>[2x]MYRTAASRARALKGVLTRSLRPARYASSSAVAETSSSTPAYLSWLSGGSRAALTSLDMPLQGVSLPPPLADKVEPSKLQITTLPNGLKIASETTPNPAASIGLYVDCGSIYEAPYFHGATHLLERMAFKSTLNRTHFRLVREIEAIGGNTSASASREQMSYTIDALKTYVPEMVEVLIDSVRNPAFLDWEVNEELRKMKVEIAELAKNPMGFLLEAIHSAGYSGPLASPLYAPESALDRLNGELLEEFMTENFTAARMVLAASGVEHEELLKVAEPLTSDLPNVPPQLAPKSQYVGGDFRQHTGGEATHFAVAFEVPGWNNEKEAVTATVLQMLMGGGGSFSAGGPGKGMHSWLYRRVLNEYQEVQSCTAFTSIFNDTGLFGIYGCSSPQFAAKAIELAAKELKDVAGGKVNQAHLDRAKAATKSAVLMNLESRMIAAEDIGRQILTYGERKPVDQFLKSVDQLTLKDIADFTSKVISKPLTMGSFGDVLAVPSYDTISSKFR;>[2x]MAMKNLLSLARRSQRRLFLTQATRSSSSFSAIDSVPASASPTALSPPPPHLMPYDHAAEIIKNKIKKLENPDKRFLKYASPHPILASHNHILSAPETRVTTLPNGLRVATESNLSAKTATVGVWIDAGSRFESDETNGTAHFLEHMIFKGTDRRTVRALEEEIEDIGGHLNAYTSREQTTYYAKVLDSNVNQALDVLADILQNSKFEEQRINRERDVILREMQEVEGQTDEVVLDHLHATAFQYTPLGRTILGPAQNVKSITREDLQNYIKTHYTASRMVIAAAGAVKHEEVVEQVKKLFTKLSSDPTTTSQLVANEPASFTGSEVRMIDDDLPLAQFAVAFEGASWTDPDSVALMVMQTMLGSWNKNVGGGKHVGSDLTQRVAINEIAESIMAFNTNYKDTGLFGVYAVAKADCLDDLSYAIMYEVTKLAYRVSDADVTRARNQLKSSLLLHMDGTSPIAEDIGRQLLTYGRRIPTAELFARIDAVDASTVKRVANKYIYDKDIAISAIGPIQDLPDYNKFRRRTYWNRY;>[2x]MLRVAGRRLFSVSQRSSTATSFVVSRDHTLSDGGGDSSSAPRSLPSADLSSYHRSLIRGFSSQVLAQGNEIGFGSEVPATVEAVKTPNSKIVYDDHNHERYPPGDPSKRAFAYFVLSGGRFVYASVLRLLVLKLIVSMSASKDVLALASLEVDLGSIEPGTTVTVKWRGKPVFIRRRTEDDIKLANSVDVGSLRDPQEDSVRVKNPEWLVVVGVCTHLGCIPLPNAGDYGGWFCPCHGSHYDISGRIRKGPAPYNLEVPTYSFLEENKLLIG;>MASFLQRLVDPRKNFLARMHMKSVSNRLRRYGLRYDDLYDPLYDLDIKEALNRLPREIVDARNQRLMRAMDLSMKHEYLPDNLQAVQTPFRSYLQDMLALVKRERAEREALGALPLYQRTIP[2x]

Protein complexes of the mitochondrial respiratory chain assemble into respiratory supercomplexes. Here we present the high-resolution electron cryo-microscopy structure of the Arabidopsis respiratory supercomplex consisting of complex I and a complex III dimer, with a total of 68 protein subunits and numerous bound cofactors. A complex I-ferredoxin, subunit B14.7 and P9, a newly defined subunit of plant complex I, mediate supercomplex formation. We propose that the main role of the plant supercomplex is to stabilize its components in the membrane.

In plants, complex III2 contains an active MPP domain protruding into the mitochondrial matrix. Complex III2 thus has a dual function in respiratory electron transport and in the maturation of proteins imported into mitochondria. In our structure of the Arabidopsis respiratory I + III2 supercomplex, subunit MPP-β of each complex III monomer contains a bound Zn ion as a cofactor for peptidase activity. The Zn is coordinated by two histidines (H141 and H145) and a glutamate (E221). In addition, the map indicates a potentially coordinating water molecule. This water molecule is known to be catalytically relevant as it performs a nucleophilic attack on the carbonyl carbon of the substrate peptide bond. However, the adjacent glycine-rich loop of subunit MPP-α is not well resolved. This loop is flexible and involved in substrate binding and product release. The weak cryo-EM density for this region would thus indicate an active MPP domain.>MTVKSQQQIIDSFKQANQDQLFQYYDSLTIDQQQEFIDQLSTIEEPAKLISTVEQAIQFSQTNSTSRNFTQLPNEQTASTLDLSKDILQNWTELGLKAIGNGEVAVLLMAGGQGTRLGSSAPKGCFNIELPSQKSLFQIQAEKILKIEQLAQQYLKSTKKPIINWYIMTSGPTRNATESFFIENNYFGLNSHQVIFFNQGTLPCFNLQGNKILLELKNSICQSPDGNGGLYKALKDNGILDDLNSKGIKHIHMYCVDNC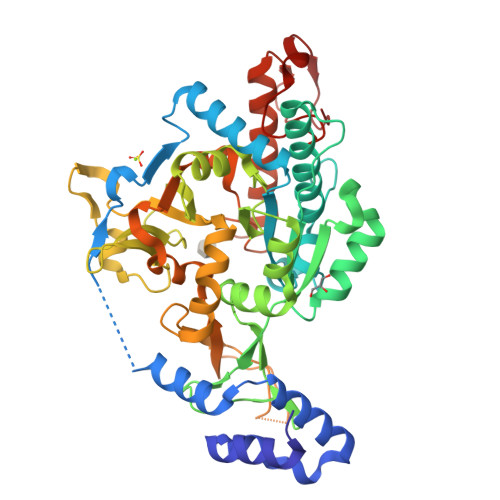LVKVADPIFIGFAIAKKFDLATKVVRKRDANESVGLIVLDQDNQKPCVIEYSEISQELANKKDPQDSSKLFLRAANIVNHYYSVEFLNKMIPKWISSQKYLPFHIAKKKIPSLNLENGEFYKPTEPNGIKLEQFIFDVFPSVELNKFGCLEVDRLDEFSPLKNADGAKNDTPTTCRNHYLERSSKWVIQNGGVIDNQGLVEVDSKTSYGGEGLEFVNGKHFKNGDII[2x]> MEQGEDITSKKDRGVLKIVKRVGNGEETPMIGDKVYVHYKGKLSNGKKFDSSHDRNEPFVFSLGKGQVIKAWDIGVATMKKGEICHLL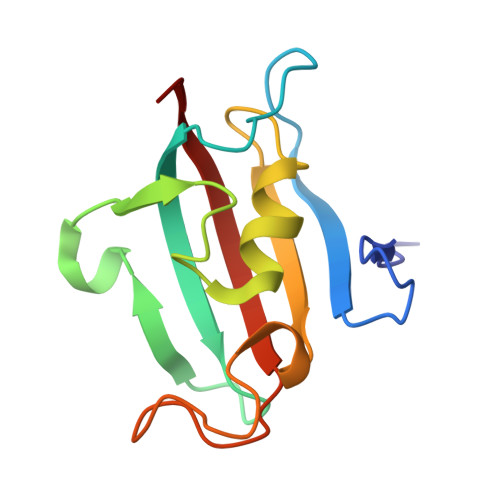CKPEYAYGSAGSLPGIPSNATLFFEIELLDFKGE> MACNKQNGVKNILITFTDCDTQEVIGPISHEQPDDTLPTYKNCAWTNTALTNGYVQRSASNATMT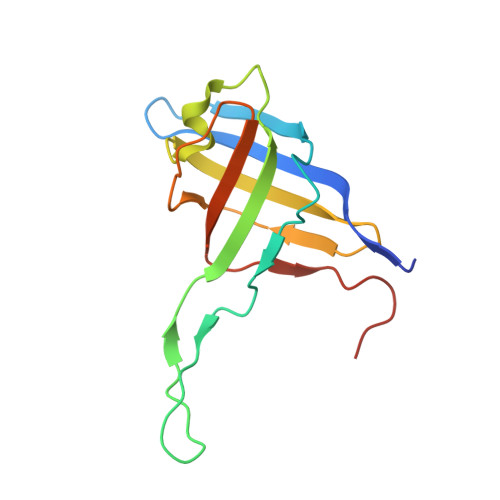LPVVRDLRVPLAFYQGCAQVDVQVEKFDGTVMTLTEGAVVEPEESDGRSVTMNIVASEIDELLPPGSLAAA>[8x]MRLKDKAVLITGAAHGIGRATLELFAKEGARLVACD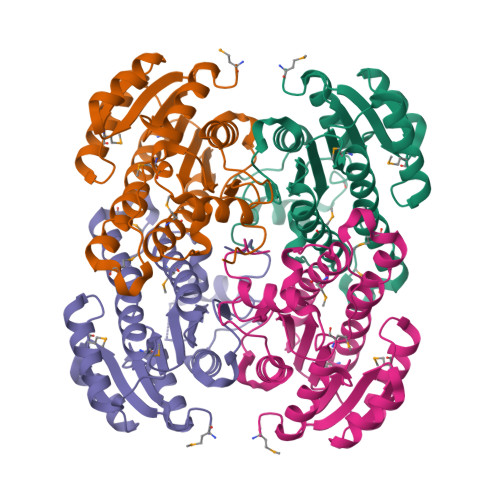IEEGPLREAAEAVGAHPVVMDVADPASVERGFAEALAHLGRLDGVVHYAGITRDNFHWKMPLEDWELVLRVNLTGSFLVAKAASEAMREKNPGSIVLTASRVYLGNLGQANYAASMAGVVGLTRTLALELGRWGIRVNTLAPGFIETRMTAKVPEKVREKAIAATPLGRAGKPLEVAYAALFLLSDESSFITGQVLFVDGGRTIGAAPA> MIAGPEALLDR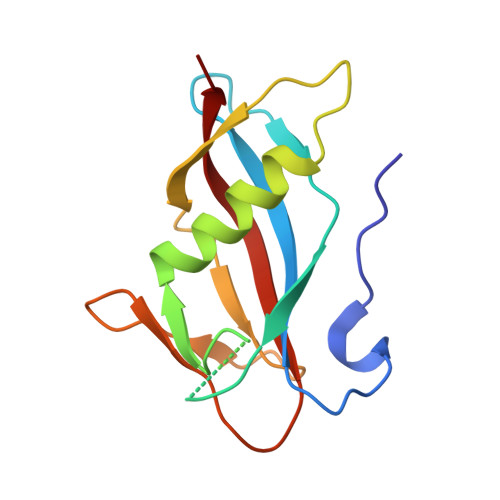PSVNNSQLVVSVAGTVEGTNQDISLKFFEIDLTSRPASKPFATDSGAMPHKLEKADLLKAIQEQLIANVHSNDDYFEVIDFASDATITDRNGKVYFADKDGSVTLPTQPVQEFLLSGHVRVRPYK> MAAGVPKIDALESLGNPLEDAKRAAAYRAVDENLKFDDHKIIGIGSGSTVVYVAERIGQYLHDPKFYEVASKFICIPTGFQSRNLILDNKLQLGSIEQYPRIDIAFDGADEVDENLQLIKGGGACLFQEKLVSTSAKTFIVVADSRKKSPKHLGKNWRQGVPIEIVPSSYVRVKNDLLEQLHAEKVDIRQGGSAKAGPVVTDNNNFIIDADFGEISDPRKLHREIKLLVGVVET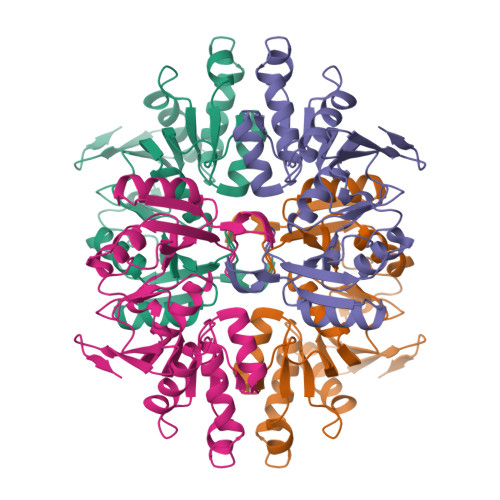GLFIDNASKAYFGNSDGSVEVTEKHHHHHH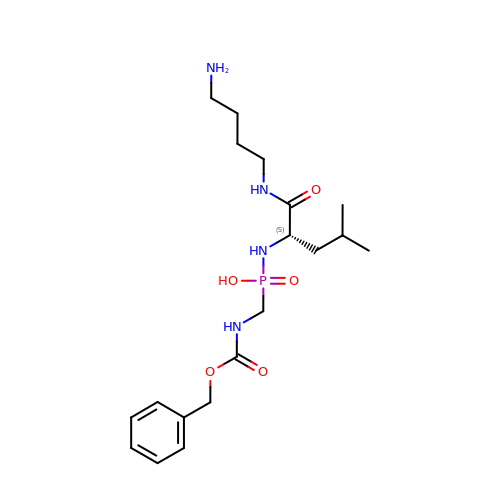~{N}-[(2~{S})-1-(4-azanylbutylamino)-4-methyl-1-oxidanylidene-pentan-2-yl]-(phenylmethoxycarbonylaminomethyl)phosphonamidic acid | C19 H33 N4 O5 P | NELYNJBBQIDLOY-KRWDZBQOSA-N>[2x]MIDLIVSQGRVADRAAWMIEGAARTARALEERYGLKGHYVGEPAPHADDDWSVALPQARETLVAVREAATESIKGDNLTVLVNNTHSVSLATLPVVAREHPDAVVLYIDGHGDFNTPETTD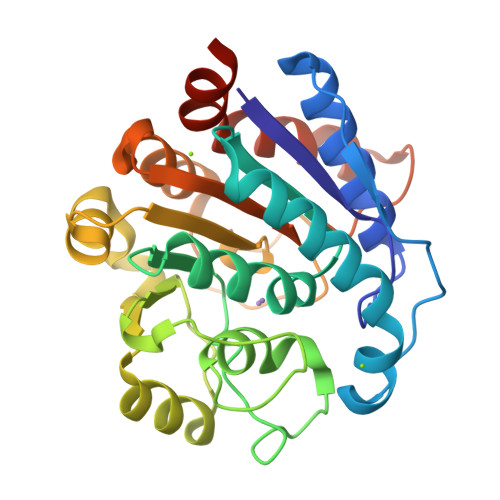TGNLHGMVLSGACGLWDSGHGAGLRPEQAVLVGSRDIDEGERELIRKAGVRVIPPGEATAQAVLDAVKDAPVWISIDWDVLEPGSIPADYTVPDGMLPAQIRAVFEAIPAERLIGVELAELNAPADSERAEQAVAVILDMVAPAFDAAAARPLEHHHHHH(1r,3r)-3-[(3-fluoropyridin-2-yl)amino]-1-methylcyclobutan-1-ol 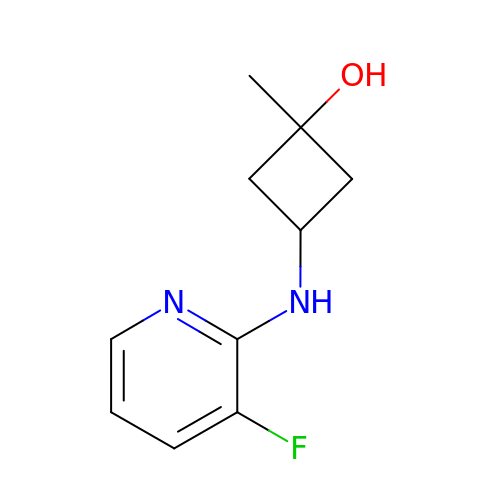| C10 H13 F N2 O | URAQAFQZSFUVGH-WKFQBHICSA-N>SMASDMEEKFREAFILFSSCSDHIEMYKFFELMNSFGIILTNDEKAALPNDINMDY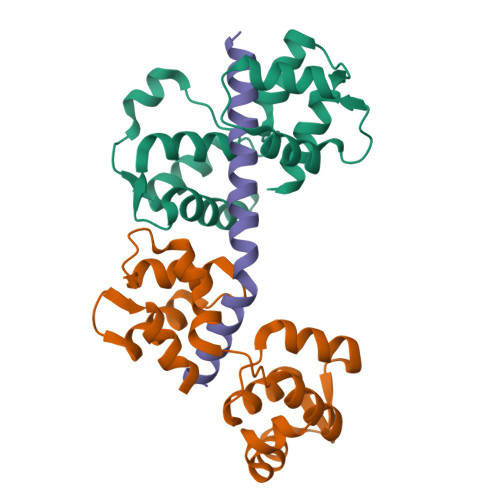WLNFAKKHYNYEQPFKHINNVNEQNTNVQIKIDNFLGIMKALDTRLTESDLNILLQITNPENKSTLNLKTVSQKLTESI[5x];>[5x]SMESVADIQQLEEKVDESDVRIYFNEKSSGGKISIDNASYNARKLGLAPSSIDEKKIKELYGDNLTYEQYLEYLSICVHDKDNVEELIKMFAHFDNNCTGYLTKSQMKNILTTWGDALTDQEAIDALNAFSSEDNIDYKLFCEDILQ;>SVEWENCVSVIEAAILKHKYKQKVNKNIPSLLRVQAHIRKKMV[5x]> LECHNQQSSQTPTTKTCSGE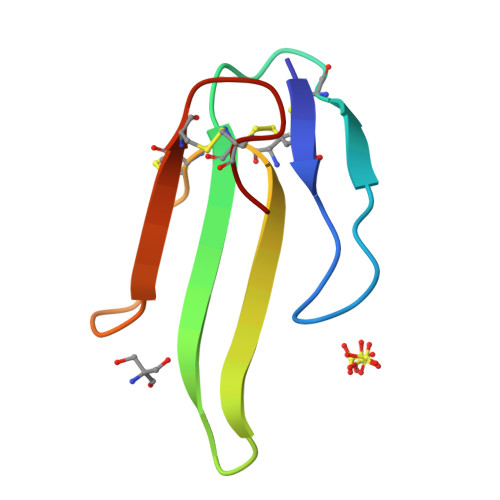TNCYKKWWSDHRGTIIERGCGCPKVKPGVNLNCCTTDRCNN> MSASVTVLWDKEIEGSNEVVKVDEMV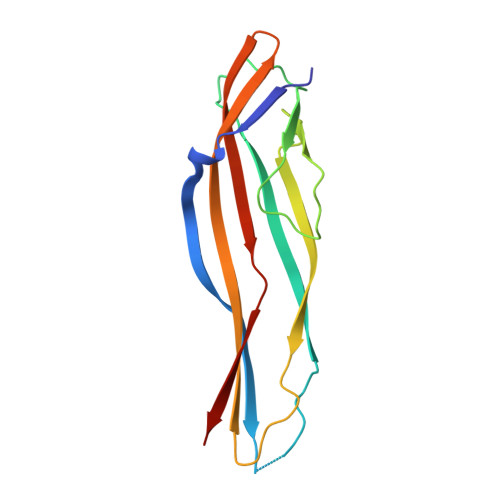ASNISNVKVEFYLKERHFDRTITHNITLPRATEVPIGTEIQLEPKHRLNGNTEPITFTYGSLESYTELSEDKVTMPEFVEPKTKLIVILTRNENITSAPVEISVGDIKETATYICQSQSGINAEVNTEPL>[4x]MSVEGLGKDFCGAIIPDNFFPIEKLRNYTQMGLIRDFAKGSAVIMPGEEITSMIFLVEGKIKLDIIFEDGSEKLLYYAGGNSLIGKLYPTGNNIYATAM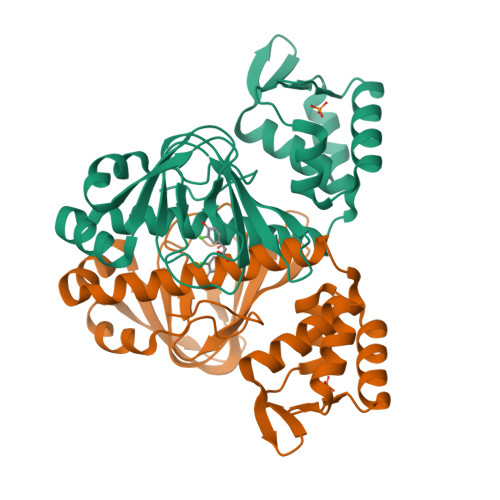EPTRTCWFSEKSLRTVFRTDEDMIFEIFKNYLTKVAYYARQVAEMNTYNPTIRILRLFYELCSSQGKRVGDTYEITMPLSQKSIGEITGVHHVTVSRVLASLKRENILDKKKNKIIVYNLGELKHLSEQTSYYSDPNSSSVDKLAAALDHH>MANLNQIQKEVSEILSDQKSMK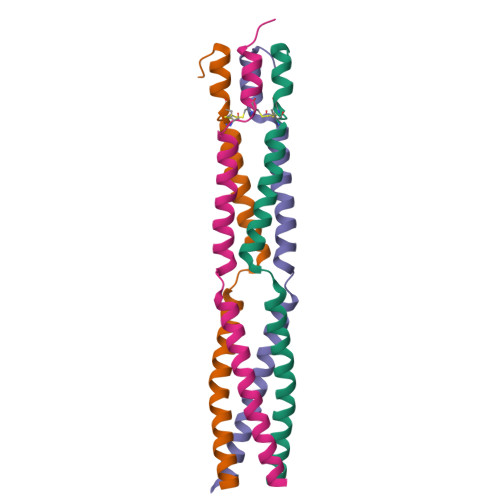ADIKAILELLGSQNPIKESLETVAAKIVNDLTKLINDCPCNKEILEALGTQPKEQLIEQPKEKGKGLNLGKYSYPNYGVGNEELGSSGNPKALTWPFKAPAGWPNQF[4x]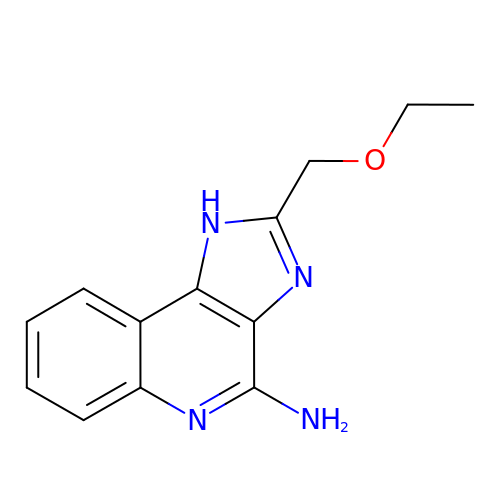2-(ethoxymethyl)-1H-imidazo[4,5-c]quinolin-4-amine | C13 H14 N4 O | DEVCLHVFELRPIU-UHFFFAOYSA-N>[12x]MSKTESYCLEDALNDLFIPETTIETILKRLTIKKNIILQGPPGVGKTFVARRLAYLLTGEKAPQRVNMVQFHQSYSYEDFIQGYRPNGVGFRRKDGIFYNFCQQAKEQPEKKYIFIIDEINRANLSKVFGEVMMLMEHDKRGENWSVPLTYSENDEERFYVPENVYIIGLMNTADRSLAVVDYALRRRFSFIDIEPGFDTPQFRNFLLNKKAEPSFVESLCQKMNELNQEISKEATILGKGFRIGHSYFCCGLEDGTSPDTQWLNEIVMTDIAPLLEEYFFDDPYKQQKWTNKLLGDSSGSHHHHHH;>[2x]MEQPVIPVRNIYYMLTYAWGYLQEIKQANLEAIPGNNLLDILGYVLNKGVLQLSRRGLELDYNPNTEIIPGIKGRIEFAKTIRGFHLNHGKTVSTFDMLNE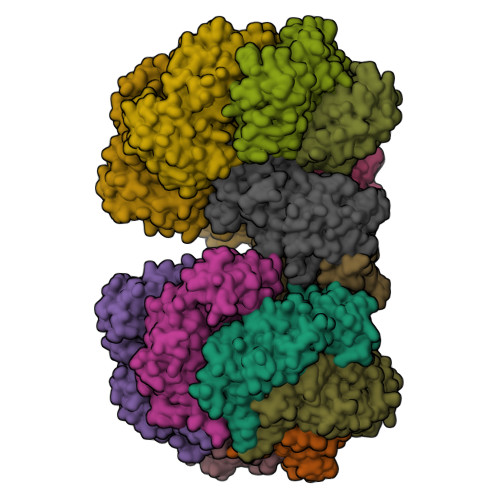DTLANRIIKSTLAILIKHEKLNSTIRDEARSLYRKLPGISTLHLTPQHFSYLNGGKNTRYYKFVISVCKFIVNNSIPGQNKGHYRFYDFERNEKEMSLLYQKFLYEFCRRELTSANTTRSYLKWDASSISDQSLNLLPRMETDITIRSSEKILIVDAKYYKSIFSRRMGTEKFHSQNLYQLMNYLWSLKPENGENIGGLLIYPHVDTAVKHRYKINGFDIGLCTVNLGQEWPCIHQELLDIFDEYLK> MKIRSQVGMVLNLDKCIGCHTCSVTCKNVWTSREGVEYAWFNNVETKPGQGFPTDWENQEKYKGGWIRKINGKLQPRMGNRAMLLGKIFANPHLPGIDDYYEPFDFDYQNLHTAPEGSKSQPIARPRSLITGERMAKIEKGPNWEDDLGGEFDKLAKDKNFDNIQKAMYSQFENTFMMYLPRLCEHCLNPACVATCPSGAIYKREEDGIVLIDQDKCRGWRMCITGCPYKKIYFNWKSGKSEKCIFCYPRIEAGQPTVCSETCVGRIRYLGVLLYDADAIERAASTENEKDLYQRQLDVFLDPNDPKVIEQAIKDGIPLSVIEAAQQSPVYKMAMEWKLALPLHPEYRTLPMVWYVPPLSPIQSAADAGELGSNGILPDVESLRIPVQYLANLLTAGDTKPVLRALKRMLAMRHYKRAETVDGKVDTRALEEVGLTEAQAQEMYRYLAIANYEDRFVVPSSHRELAREAFPEKNGCGFTFGDGCHGSDTKFNLFNSRRIDAIDVTSKTE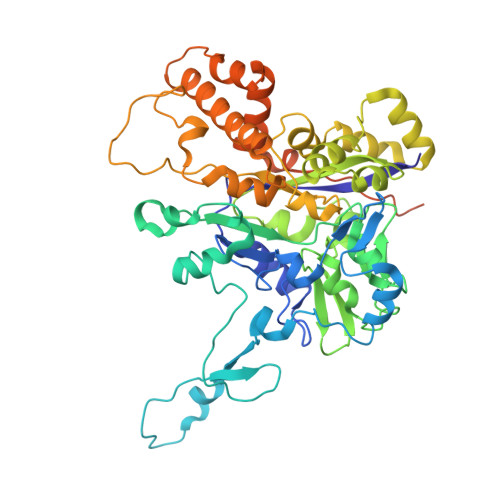PHP N-ACETYL-N-[1-(1,1'-BIPHENYL-4-YLMETHYL)-2-OXOAZEPAN-3-YL]-3,4-DIPHOSPHONOPHENYLALANINAMIDE | C30 H35 N3 O9 P2 | 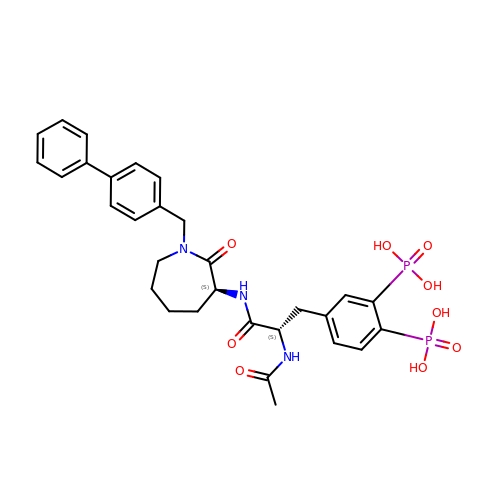WCMLXBUNHNAMNH-UIOOFZCWSA-N>MADIPNSDKIACGRKPMFCEIIKLANRKRLIFNTTDERV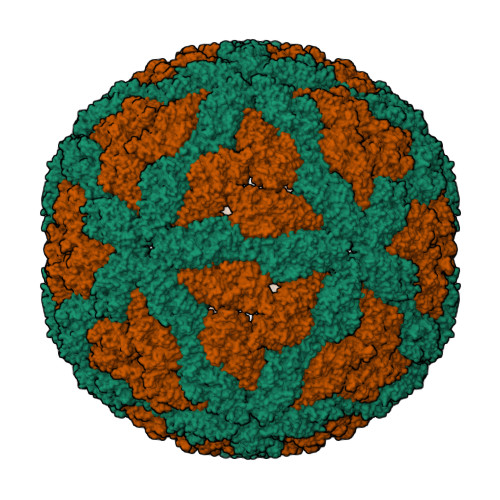YDARLNYCSTADSTVQADCHIYWRLKLRRTDAVFEEYTGQGYSLDTAAYPQQYTDIIRGYYSKHVSSSLAANTQHFVNVLAMLRHAGACIAHYCMTGKIDFDILSKKKHKNKEVVTLSNADSLSFLPHSALYLPSPLRASDPEIFNMLYLLGCACDASIAMDNISNTSGAAKYSMPHYNPLQLSHALHVTIFYMLSLMDSCGYGDDAVLALTSGLHSVTTVIAHSDEGGITRDALRELSYTQPYGTMPVPIAGYFQHINVLFTTQPAWDQFAGIWDYVILATAALVHLSDPGMTVNDVTYPTTLTTKVATVDGRNSDLAAQMMHSATRFCDIFVENLSTFWGVVANPDGNASQALLHAFNIVACAVEPNRHLEMNVMAPWYWVESSALFCDYAPFRSPISSAGYGPQCVYGARLVLAATNSLEFTGEAGDYSAYRFEWTTMRHNPLFNILNKRVGDGLANVDFRLRPFNEWLLEGQPSRRSCNSAGHGTPTATCSHKTPNHDTLDEYIWGSTSCDLFHPAELTSYTAVCVRFRNYLSGADGDVRILNTPTREVIEGNVVTRCDGIRCLDSNKRIQHVPEVARRYCMMARYLAQARTFGALTIGDDIIRGFDKVEKIVKMHKSNNRLDQMPLIDVTGLCQPMIETSTVRASTTTRIDPNKLAAATARVELPLAPRCTSSLIPSSDTVPEPEPQVGEPGDNGGCAPDLGTGGGSGIEGRGSMDIGDPNSVQALARLQASSVDKLAAALE[2x]> GKTNDWLDFDQLAEEKVRDALKPPSMYKVILVNDDYT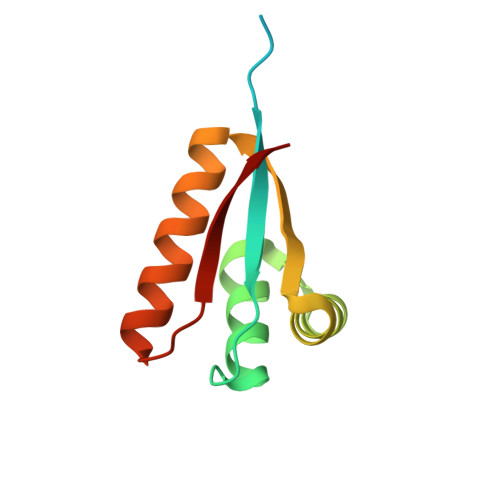PMEFVIDVLQKFFSYDVERATQLMLAVHYQGKAICGVFTAEVAETKVAMVNKYARENEHPLLCTLEKA> MCDLRRPAAGGMMDLAYVCEWEKWSKSTHCPSVPLACAWSCRNLIAFTMDLRSDDQDLTRMIHILDTEHPWDLHSIPSEHHEAI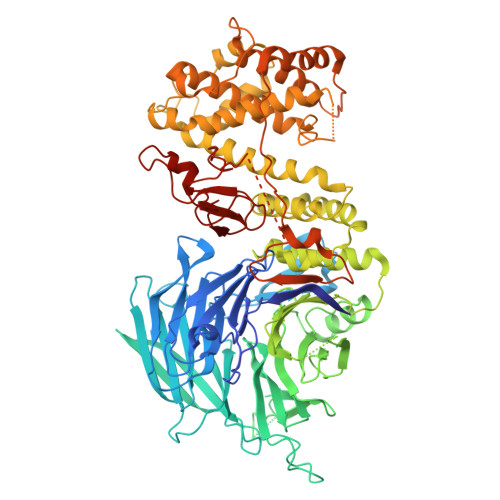TCLEWDQSGSRLLSADADGQIKCWSMADHLANSWESSVGSLVEGDPIVALSWLHNGVKLALHVEKSGASSFGEKFSRVKFSPSLTLFGGKPMEGWIAVTVSGLVTVSLLKPSGQVLTSTESLCRLRGRVALADIAFTGGGNIVVATADGSSASPVQFYKVCVSVVSEKCRIDTEILPSLFMRCTTDLNRKDKFPAITHLKFLARDMSEQVLLCASSQTSSIVECWSLRKEGLPVNNIFQQISPVVGDKQPTILKWRILSATNDLDRVSAVALPKLPISLTNTDLKVASDTQFYPGLGLALAFHDGSVHIVHRLSLQTMAVFYSSAAPRPVDEPAMKRPRTAGPAVHLKAMQLSWTSLALVGIDSHGKLSVLRLSPSMGHPLEVGLALRHLLFLLEYCMVTGYDWWDILLHVQPSMVQSLVEKLHEEYTRQTAALQQVLSTRILAMKASLCKLSPCTVTRVCDYHTKLFLIAISSTLKSLLRPHFLNTPDKSPGDRLTEICTKITDVDIDKVMINLKTEEFVLDMNTLQALQQLLQWVGDFVLYLLASLPNQGSLLRPGHSFLRDGTSLGMLRELMVVIRIWGLLKPSCLPVYTATSDTQDSMSLLFRLLTKLWICCRDEGPASEPDEALVDECCLLPSQLLIPSLDWLPASDGLVSRLQPKQPLRLQFGRAPTLPGSAATLQLDGLARAPGQPKIDHLRRLHLGACPTEECKACTRCGCVTMLKSPNRTTAVKQWEQRWIKNCLCGGLWWRVPLSYP Long-term immune evasion by the African trypanosome is achieved through repetitive cycles of surface protein replacement with antigenically distinct versions of the dense Variant Surface Glycoprotein (VSG) coat. The mature VSG proteins are attached to the cell surface by a GPI-anchor, and consist of two main regions: (1) a large, N-terminal domain (NTD) of roughly 300–400 amino acids that is most distal to the membrane and (2) a smaller, membrane-proximal C-terminal domain (CTD) spanning 80–120 amino acids beneath the NTD that harbors the GPI-anchor. Therefore, at the heart of antigenic variation in the African trypanosome are the NTDs of the VSGs. These large subdomains are elongated folds centered on a three-helix bundle scaffold.

VSG11 and VSG615 are related to VSG3 (the topologically-similar class of monomer/trimers with O-linked glycan PTMs), denoted as class B or N4 in the literature. NTD structures of VSG11 and VSG615 were solved to 1.23Å and 3.2Å resolution, respectively. Both reveal a fold similar to VSG3 as well as the presence of O-linked glycans on the top surface of the protein–one observed on VSG11 and two on VSG615. In addition, alignments of the VSG11WT-Iodine crystal form with the VSG11WT-Oil form show that the second helix of the three-helix bundle displays a significant conformational change in the region near the middle of the bundle, the helix becoming disordered and forming a random coil in one monomer while keeping helical structure in the other.

> NIGTGDNVLHRAALCGIIELAGKRAKLETALPNFQNELNSILELNMTAAEPTWLDQFRDKDDRSKPRDLTKQPLPKDTNWADHWTAWAKAALPLLNDETHQAKLKEYKLAGLQPEKLERARNTIRRLTAEAVAKAQDPTVAESTADLTTEEDLQKQINQAVYSKDTEPDDDFNGYTAFEGKASTNRQTICGSAVAGSKATNAMDALFCVCADDRTNGADAGKACVAGTAPGTGWNPGVTATPTGTMLQKVRKLCNTHGKTTLSAAAIEGRLTAVGNLLTRGSATSILGSFLATDCSGDQGSGMCVAYTEVTDAKGTPTKDIPWMQKLDSVRIKLQKHERAVEKLGKPQHDLKTILTLAKDPAYLQLASVGTRHLETTKQRVSNEQGKTQQTQQTCEQYNNKKNDCVKTGVCKWEE>[2x]MALLTAAARLFGAKNASCLVLAARHASASSTNLKDILADLIPKEQARIKTFRQQHGNTVVGQITVDMMYGGMRGMKGLVYETSVLDPDEGIRFRGYSIPECQKMLPKAKGGEEPLPEG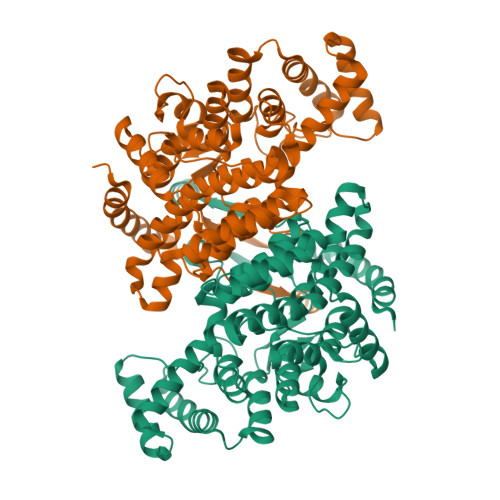LFWLLVTGQIPTEEQVSWLSKEWAKRAALPSHVVTMLDNFPTNLHPMSQLSAAITALNSESNFARAYAEGIHRTKYWELIYEDCMDLIAKLPCVAAKIYRNLYREGSSIGAIDSKLDWSHNFTNMLGYTDAQFTELMRLYLTIHSDHEGGNVSAHTSHLVGSALSDPYLSFAAAMNGLAGPLHGLANQEVLVWLTQLQKEVGKDVSDEKLRDYIWNTLNSGRVVPGYGHAVLRKTDPRYTCQREFALKHLPHDPMFKLVAQLYKIVPNVLLEQGKAKNPWPNVDAHSGVLLQYYGMTEMNYYTVLFGVSRALGVLAQLIWSRALGFPLERPKSMSTDGLIKLVDSK>[4x]HVTQSSSAITPGQTAELYPGDIKSVLLTAEQIQARIAELGEQIGNDYRELSATTGQDLLLITV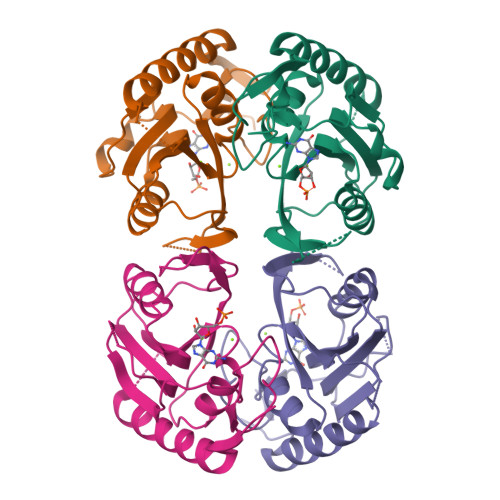LKGAVLFVTDLARAIPVPTQFEFMAVSSYGSSTSSSGVVRILKDLDRDIHGRDVLIVEDVVDSGLTLSWLSRNLTSRNPRSLRVCTLLRKPDAVHANVEIAYVGFDIPNDFVVGYGLDYDERYRDLSYIGTLDPRVYQ>MGFGELKEEWRGEVVHLSWSPRAFLLKNFLSDEECDYIVEKARPKMVKSSVVDNESGKSVDSEIRTSTGTWFAKGEDSVISKIEKRVAQVTMIPLENHEGLQVLHYHDGQKYEPHYDYFHDPVNAGPEHGGQRVVTM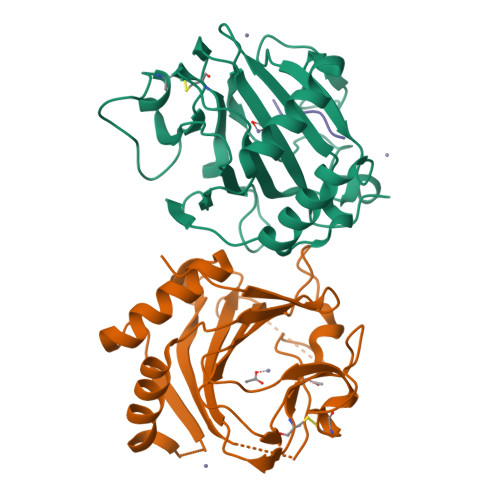LMYLTTVEEGGETVLPNAEQKVTGDGWSECAKRGLAVKPIKGDALMFYSLKPDGSNDPASLHGSCPTLKGDKWSATKWIHVAPIGGRH[4x];>[2x]SPSPSPSPSP>MQVKPCTPEFYQTHFQLAYRLQSRPRGLALVLSNVHFTGEKELEFRSGGDVDHSTLVTLFKLLGYDVHVLCDQTAQEMQEKLQNFAQLPAHRVTDSCIVALLSHGVEGAIYGVDGKLLQLQEVFQLFDNANCPSLQNKPKMFFIQACRGDETDRGVDQQD[2x];>GKEKLPKMRLPTRSDMICGYACLKGTAAMRNTKRGSWYIEALAQVFSERACDMHVADMLVKVNALIKDREGYAPGTEFHRCKEMSEYCSTLCRHLYLFPG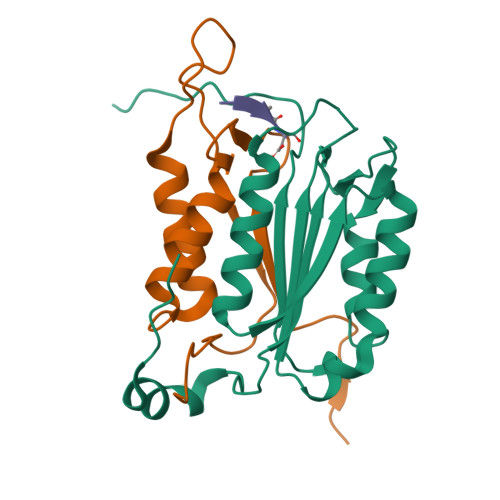HPPTLEHHHHHH[2x];>XDVAD[2x]> MSSVTWAPGNYPSTRRSDHVDTYQSASKGEVPVPDPYQWLEESTDEVDKWTTAQADLAQSYLDQNADIQKLAEKFRASRNYAKFSAPTLLDDGHWYWFYNRGLQSQSVLYRSKEPALPDFSKGDDNVGDVFFDPNVLAADGSAGMVLCKFSPDGKFFAYAVSHLGGDYSTIYVRSTSSPLSQASVAQGVDGRLSDEVKWFKFSTIIWTKDSKGFLYQRYPARERHEGTRSDRNAMMCYHKVGTTQEEDIIVYQDNEHPEWIYGADTSEDGKYLYLYQFKDTSKKNLLWVAELDEDGVKSGIHWRKVVNEYAADYNIITNHGSLVYIKTNLNAPQYKVITIDLSKDEPEIRDFIPEEKDAKLA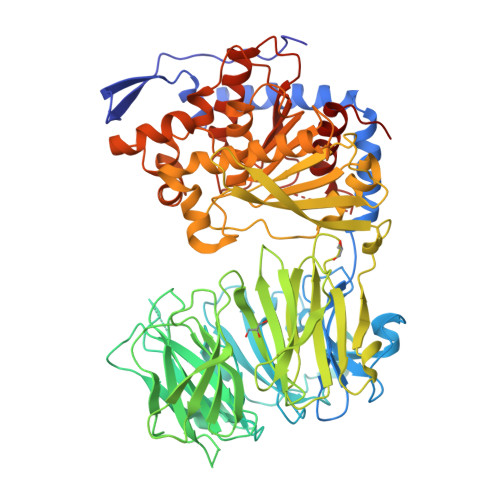QVNCANEEYFVAIYKRNVKDEIYLYSKAGVQLTRLAPDFVGAASIANRQKQTHFFLTLSGFNTPGTIARYDFTAPETQRFSILRTTKVNELDPDDFESTQVWYESKDGTKIPMFIVRHKSTKFDGTAAAIQYGYGGFATSADPFFSPIILTFLQTYGAIFAVPSIRGGGEFGEEWHKGGRRETKVNTFDDFIAAAQFLVKNKYAAPGKVAINGASNGGLLVMGSIVRAPEGTFGAAVPEGGVADLLKFHKFTGGQAWISEYGNPSIPEEFDYIYPLSPVHNVRTDKVMPATLITVNIGDGRVVPMHSFKFIATLQHNVPQNPHPLLIKIDKSWLGHGMGKPTDKNVKDAADKWGFIARALGLELKTVE> GGSMGKTADNHGPVRSETAREGRENQVYSPVTGARLVAGCICLTPDKKQVLMITSSAHKKRWIVPAGGVEKDEPNYETTAQRETWEEAGCIGKIVANLGTVEDMRPPKDWNKDIKQFENSRKDSEVAKHPPRTEFHFYELEIENLLDKFPECHKRHRKLYSYTEAKQNLIDAKRPELLEALNRSAIIKDDK

The yeast diadenosine and diphosphoinositol polyphosphate phosphohydrolase DDP1 is a Nudix enzyme with pyrophosphatase activity on diphosphoinositides, dinucleotides, and polyphosphates. ScDDP1, like its human orthologs, adopts the canonical Nudix fold showing two β sheets flanked by helices. The active site lies in the crevice situated between both β sheets. The longest helix (α-1) contains the Nudix box (GX5EX7REUXEEXGU), which displays a β-loop-helix-loop structure that binds the Mg2+ ions involved in diphosphate moiety orientation and catalysis.

Our analysis provided very interesting results: First, three mutants show prominent increases in thermal stability in the free state (K63A, R171S, and Δnose) as compared to the wild type. Both basic residues are very close to each other and other positive charges. Therefore, it seems that removing the positive charges relieves the tension in this highly electropositive active site, especially those for Lys63, the mutation of which apparently increased the thermal stability by almost 12°C. As mentioned, Lys63 is not conserved in HsDIPPs; however, it is conserved in MsMutT1 enzyme. Although ScDDP1 failed to crystallize in the absence of ligands or analogs, the stabilized ScDDP1-K63A allowed us to solve the structure of DDP1 in the unbound form, revealing that no important structural changes are seen in the active site upon binding beyond minor side chain accommodations of a few basic residues. A retreat from the active site of the mobile Ser-loop (52-SSA) involved in phosphate binding is also observed in this mutant. Some kind of activity decrease is in concordance with a less efficient polyphosphate binding being more evident in the case of K63A mutant.The kallikrein (KLK) gene family is the largest protease gene cluster in the human genome and encodes 15 serine proteases that have sequence identity varying from 40–80%, with a high degree of structural similarity around the active site1. KLK4 is predominantly expressed in basal and secretory cells of the prostate gland with lower levels of expression in a number of tissues including breast, ovaries, thyroid, testis and developing teeth. Over-expression of KLK4 has been documented in malignant prostate, ovarian and breast tumors and is associated with metastasis, and mechanisms underpinning resistance to androgen deprivation therapy. In order to investigate further both direct and indirect mechanisms of KLK4 inhibition here we describe the structures of KLK4 in complex with SFTI-1, an engineered SFTI-1 variant, and with nickel (KLK4-Ni).

KLK4 displayed the highest activity for the FVQR-p-nitroanilide (pNA) substrate, with P4 and P2 residues affecting activity the most. This sequence was grafted onto the SFTI-1 scaffold with the retention of the cysteine, creating SFTI-1FCQR (SFTI-1 substituted with Phe2, Gln4 and Arg5), and resulted in a 18-fold increased inhibition of KLK4 (Ki = 3.59 nM). To investigate the structural basis for increased potency, we solved the crystal structure of a KLK4-SFTI-1FCQR complex to 1.3 Å resolution. Compared with KLK4-SFTI-1 there is an overall increase in the buried surface area and number of protease-inhibitor interactions, consistent with the increased inhibitory potency of SFTI-1FCQR. Binding can be mainly attributed to improved interactions at mutated residues P4, P2 and P1. At the S4 site, the KLK4-SFTI-1FCQR structure shows conformational selection and/or induced fit upon binding, where the replacement of Arg at P4 with Phe is associated with a movement of loop VI towards the inhibitor, suggesting an improved interaction. Deep in the S2 pocket, the KLK4-SFTI-1FCQR structure shows an interaction between Gln4NE of SFTI-1FCQR and Tyr94O of KLK4. While there is still a requirement for hydrophobic interactions in the shallow of the S2 pocket, this observation provides a structural explanation for why the polarity of Gln is desirable in the S2 pocket, and goes some way to explaining the preference for Gln>Val>Leu>Thr at the S2 subsite previously reported. There are also several secondary effects that contribute to improved binding at unchanged SFTI-1 residues, notably P2′ and Phe12. These secondary effects are seen as unbroken density for Pro13 and Asp14, which can now be fully resolved, in contrast to KLK4-SFTI-1. The KLK4-SFTI-1FCQR structure shows an alternative loop III conformation to those obtained in the KLK4-Ni and KLK4-SFTI-1 structures. This single, less-frustrated conformation was maintained throughout all simulations of KLK4 with SFTI-1FCQR.

> IINGEDCSPHSQPWQAALVMENELFCSGVLVHPQWVLSAAHCFQNSYTIGLGLHSLEADQEPGSQMVEASLSVRHPEYNRPLLANDLMLIKLDESVSESDTIRSISIASQCPTAGNSCLVSGWGLLANGRMPTVLQCVNVSVVSEEVCSKLYDPLYHPSMFCAGGGQDQKDSCNGDSGGPLICNGYLQGLVSFGKAPCGQVGVPGVYTNLCKFTEWIEKTVQA;> GFCQRSIPPICFPD>[8x]LSSSPSEILQELGKGSTHPQPGVSPPAAPAAPGPKDGPGETDAFGNSEGKELVASGENKIKQGLLPSLEDLLFYTIAEGQEKIPVHKFITALKSTGLRTSDPRLKECMDMLRLTLQTTSDGVMLDKDLFKKCVQSNIVLLTQAFRRKFVIPDFMSFTSHIDELYESAKKQSGGKVADYIPQLAKFSPDLWGVSVCTADGQRHSTGDTKVPFCLQSCVKPLKYAIAVNDLGTEYVHRYVGKEPSGLRFNKLFLNEDDKPHNPMVNAG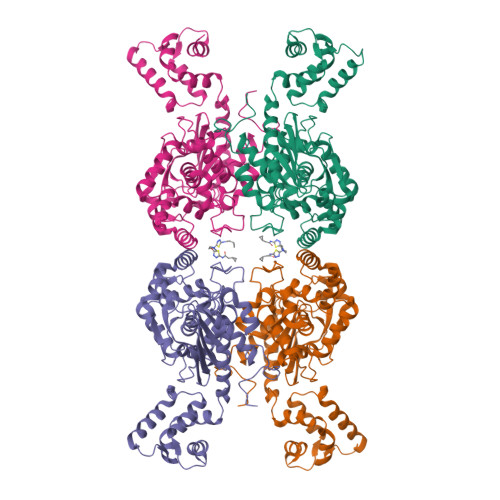AIVVTSLIKQGVNNAEKFDYVMQFLNKMAGNEYVGFSNATFQSERESGDRNFAIGYYLKEKKCFPEGTDMVGILDFYFQLCSIEVTCESASVMAATLANGGFCPITGERVLSPEAVRNTLSLMHSCGMYDFSGQFAFHVGLPAKSGVAGGILLVVPNVMGMMCWSPPLDKMGNSVKGIHFCHDLVSLCNFHNYDNLRHFAKKLDPRREGGDQRHSFGPLDYESLQQELALKETVWKKVSPESNEDISTTVVYRMESLGEKS>GTGDGSMPATVAELQAEIAAWIHPLNPDRRPGGTIAKLLEEIGELIASDRAHDPLEVADVLILALDLATLLGVDVTEAIRAKLAINRARSWARADNGAMRHIPGSDTPSFP[4x]

Cyanophage S-2L is known to profoundly alter the biophysical properties of its DNA by replacing all adenines (A) with 2-aminoadenines (Z), which still pair with thymines but with a triple hydrogen bond. It was recently demonstrated that a homologue of adenylosuccinate synthetase (PurZ) and a dATP triphosphohydrolase (DatZ) are two important pieces of the metabolism of 2-aminoadenine, participating in the synthesis of ZTGC-DNA. We now propose a complete 2-aminoadenine metabolic pathway for cyanophage S-2L and related Siphoviridae and Podoviridae phages. The post-infection composition of cellular dNTP pool is heavily altered: dATP is eliminated and replaced by dZTP, which is created in turn from dGTP.

Purified MazZ of cyanophage S-2L is capable of removing two terminal phosphates from a nucleoside triphosphate. Its preferential substrates, dGTP and GTP, are rapidly dephosphorylated to dGMP and GMP, respectively. We obtained crystals of MazZ and solved its structure, bound to the dephosphorylation product of dGTP and catalytic Mn2+ ions, at 1.43 Å resolution. Contrary to other members of the all-α NTP-PPase superfamily, each MazZ protein chain has two additional β-strands at its C-terminus. Together, they form a homotetramer with a typical MazG-HisE fold: to our knowledge, it is the first time that the fold is recognized as identical for all MazG, MazG-like and HisE enzymes, despite the number of determined structures. The whole MazZ tetramer constitutes the asymmetric unit. The dGDP intermediate observed in crystallo is almost completely buried inside the enzyme, except for the solvent-exposed β-phosphate next to which we found three catalytic Mn2+ ions. The closest residue to guanine’s O6 is N20, through its amide nitrogen at 3.2 Å; the 2-amino group is only 3.0 Å away from the carboxyl group of D60. Altogether, the specificity of MazZ emerges from the cavity volume matching guanine’s shape and its charge compatibility. Ion A is coordinated by residues E34, E35 and E38; ion B by E50 and D53; and ion C by E38 and E50.V1 is a part of an ion pump V-ATPase, which transports cations across the membrane by ATP-hydrolysis-driven rotation. V1 comprises a rotor composed of the D and F subunits, and a stator, a hexameric ring, composed of three A subunits and three B subunits. However, the details of their sequences and structures are different, resulting in two different interfaces between the A and B subunits in the A3B3 hexameric ring: a catalytic interface, at which the A subunit has an ATP-hydrolysis catalytic site; and a non-catalytic interface, at which the B subunit has a pseudo-active site, which has evolutionally lost the ATP-hydrolysis or even binding ability. We used computational design to restore the lost ATP-binding ability of the pseudo-active site in the B subunit of a rotary molecular motor, V1-ATPase.

Next, the nucleotide-free crystals were incubated for 5 h in the presence of ADP by gradually increasing the ADP concentration to 10 mM, and the resulting structure, A3(De)3_(ADP·Pi)1cat(ADP)2cat,2non-cat, was solved at 3.2 Å resolution. In A3(De)3_(ADP·Pi)1cat(ADP)2cat,2non-cat, each of the three catalytic sites is occupied by an ADP (one of the sites has an ADP with a possible Pi) and each of the two designed sites out of the three is occupied by an ADP. This structure proved that the designed site has nucleotide-binding ability: the designed P-loop (green) exhibits typical backbone geometry and accurately binds to the phosphate group of an ADP. However, interestingly, the ADP is bound in the opposite direction to the design: although the β phosphate is located at the same position as in the design model, the α phosphate is located at the position of the γ phosphate in the design model, and the sugar and base are at the interface with the A subunit. Note that, like naturally occurring P-loops, the designed P-loop grabs two phosphates. The observed unintended ATP-binding mode probably originated because we designed the binding site only in the monomer B subunit without considering the A subunit. The designed P-loop (green) firmly grabs the phosphate group of ADP. The sugar and base of ADP were found at the interface with the A subunit (cyan).

>[3x]SSGMQIGKIIKVSGPLVMAENMSEASIQDMCLVGDLGVIGEIIEMRQDVASIQVYEETSGIGPGEPVRSTGEALSVELGPGIISQMFDGIQRPLDTFMEVTQSNFLGRGVQLPALDHEKQWWFEATIEEGTEVSAGDIIGYVDETKIIQHKIMVPNGIKGTVQKIESGSFTIDDPICVIETEQGLKELTMMQKWPVRRGRPIKQKLNPDVPMITGQRVIDTFFPVTKGGAAAVPGPFGAGKTVVQHQIAKWSDVDLVVYVGCGERGNEMTDVVNEFPELIDPNTGESLMERTVLIANTSNMPVAAREASIYTGITIAEYFRDMGYDVAIMADSTSRWAEALREMSGRLEEMPGDEGYPAYLGSRLAEYYERSGRVIALGSDQREGSITAISAVSPSGGDISEPVTQNTLRVVKVFWGLDSSLAQKRHFPSINWIQSYSLYSTEVGRYMDQILQQDWSDMVTEGMRILQEEEQLNEIVRLVGIDSLSDNDRLTLEVAKSIREDYLQQNAFDDVDTFTSREKQFNMLKVILTFGKEARKALSLGAYFNEIMEGTVAVRERISRSKYIPEEELAKISSINEEIKETIQLIVSEGGMTDD;>MIKEYRTIKEVVGPLMAVEKVSGVKYEELIEVRMQNGEIRRGQVLEVQEDKAMVQIFEGTSGINLKNSSVRFLGHPLQLGVSEDMIGRVFDGLGRPKDNGPEILPEKYLDINGEVINPIARDYPDEFIQTGISAIDHLNTLVRGQKLPVFGPPGAGKSALAAQIARQATVLDSSDDFAVVFAAIGITFEEAEFFMEDFRQTGAIDRSVMFMNLANDPAIERIATPRMALTAAEYLAYEKGMHVLVIMEDMTNYAEALREISAARREVPGRRGYPGYLYTNLATLFERAGRIRGLKGSVTQIPILTMPEDDKTHPIPDLTGYITEGQIILTRELYKSGISPPIDVLPSLSRLKDKGTGAGKTREDHAATMNQLFAAYAQGKQAKELAVVLGESALSDIDKIYAKFAERFENEYVNQGFYTNRTITETLDLGWELLAMLPRTELKRIKDDLLDKYLPEGK[3x]>[3x]MESKRLDNAALAAGISPNYINAHGKPQSISAETKRRLLDAMHQRTATKVAVTPVPNVMVYTSGKKMPMVVEGSGEYSWLLTTEEGTQYKGHVTGGKAFNLPTKLPEGYHTLTLTQDDQRAHCRVIVAPKRCYEPQALLNKQKLWGACVQLYTLRSEKNWGIGDFGDLKAMLVDVAKRGGSFIGLNPIHALYPANPESASPYSPSSRRWLNVIYIDVNAVEDFHLSEEAQAWWQLPTTQQTLQQARDADWVDYSTVTALKMTALRMAWKGFAQRDDEQMAAFRQFVAEQGD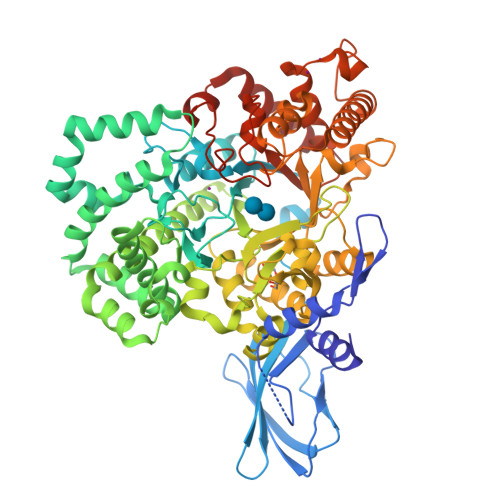SLFWQAAFDALHAQQVKEDEMRWGWPAWPEMYQNVDSPEVRQFCEEHRDDVDFYLWLQWLAYSQFAACWEISQGYEMPIGLYRDLAVGVAEGGAETWCDRELYCLKASVGAPPDILGPLGQNWGLPPMDPHIITARAYEPFIELLRANMQNCGALRIDHVMSMLRLWWIPYGETADQGAYVHYPVDDLLSILALESKRHRCMVIGEDLGTVPVEIVGKLRSSGVYSYKVLYFENDHEKTFRAPKAYPEQSMAVAATHDLPTLRGYWECGDLTLGKTLGLYPDEVVLRGLYQDRELAKQGLLDALHKYGCLPKRAGHKASLMSMTPTLNRGLQRYIADSNSALLGLQPEDWLDMAEPVNIPGTSYQYKNWRRKLSATLESMFADDGVNKLLKDLDRRRRSAHHHHHH> MLGLWGQRLPAAWVLLLLPFLPLLLLAAPAPHRASYKPVIVVHGLFDSSYSFRHLLEYINETHPGTVVTVLDLFDGRESLRPLWEQVQGFREAVVPIMAKAPQGVHLICYSQGGLVCRALLSVMDDHNVDSFISLSSPQMGQYGDTDYLKWLFPTSMRSNLYRICYSPWGQEFSICNYWHDPHHDDLYLNASSFLALINGERDHPNATVWRKNFLRVGHLVLIGGPDDGVITPWQSSFFGFYDANETVLEMEEQLVYLRDSFG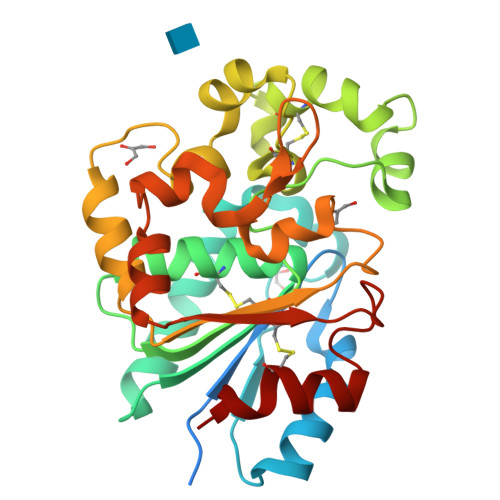LKTLLARGAIVRCPMAGISHTAWHSNRTLYETCIEPWLS>MDYLFKLLLIGDSGVGKTCVLFRFSEDAFNSTFISTIGIDFKIRTIELDGKRIKLQIWDTAGQERFRTITTAYYRGAMGIMLVYDITNEKSFDNIRNWIRNIEEHASADVEKMILGNKCDVNDKRQVSKERGEKLALDYGIKFMETSAKANINVENAFFTLARDIKAKMDKKHHHHHH[2x]

Upon attachment to their target membranes, Rab GTPases act as molecular switches that are activated by a GEF that catalyzes the exchange of the bound guanosine-5′-diphosphate (GDP) for the more abundant guanosine-5′-triphosphate (GTP). Once active, the GTP-bound Rab can interact with specific effector proteins which mediate a variety of downstream functions including binding to cargoes, enabling vesicle formation and promoting vesicle fusion to target membranes. Rabs are inactivated by GAPs that promote the hydrolysis of GTP to GDP and the inactive Rab is then relocalized to the cytosol. Structural analysis of Rab8A revealed that the PINK1-regulated Ser111 site lies within a short stretch of amino acids within the C-terminal region termed the RabSF3 motif (see Supplementary Figure S3 for a structural depiction of Rab regions and position of Ser111 and Thr72 residues).

To understand the mechanism by which Ser111 phosphorylation impacts on its interactions with its GEF, GAP and LRRK2, we solved the structure of pSer111-Rab8A. Employing genetic code expansion technologies for the incorporation of pSer65 into Ubiquitin, we were able to produce pSer111-Rab8A in the inactive GDP-bound conformation (pSer111-Rab8A:GDP) and the active GTP-bound conformation (pSer111-Rab8A:GppNHp) with a yield of 0.15 mg/l of bacterial culture. Phosphorylated Rab8A exhibits a typical small GTPase fold with highly flexible Switch regions in the GDP-bound form, and well-defined structured Switch regions in the GppNHp-bound form. The pSer111 residue is located C-terminal of helix α3 in a loop above the Switch II region (α2). The superimposed structures of pSer111-Rab8A and WT-Rab8A showed that the phosphorylation at Ser111 does not impact the overall structure of Rab8A. The phosphorylation at Ser111 did not induce any major changes in the structure of Rab8A, nor in Rab1B, despite impacting on GEF/GAP interactions. To determine whether Ser111 phosphorylation was mediating specific effects via the Switch II domain we determined the binding affinity of WT- and pSer111-Rab8A GppNHp-bound forms with the effector Mical-1, which binds outside the Switch II domain. Using ITC, we obtained a KD value of 923 nM for the binding affinity of WT-Rab8A and Mical-1, and a KD of 913 nM for pSer111 Rab8A with Mical-1, suggesting that the phosphorylation at Ser111 has no effect on Rab8-Mical-1 effector interaction. Furthermore, we did not detect any influence of Ser111 phosphorylation on the interaction with the effector Mical-1 because the Switch II region (α2) of Rab8A is not part of the Mical-1 binding site. Strikingly, we found that the ability of LRRK2 [G2019S] to phosphorylate pSer111-Rab8A:GDP was disrupted (compared with WT-Rab8A:GDP) and a similar reduction was determined for pSer111-Rab8A:GppNHp (compared with WT-Rab8A:GppNHp).>[2x]VTDLAGTTRLLRAQGVTAPAGFRAAGVAAGIKASGALDLALVFNEGPDYAAAGVFTRNQVKAAPVLWTQQVLTTGRLRAVILNSGGANACTGPAGFADTHATAEAVAAALSDWGTETGAIEVAVCSTGLIGDRLPMDKLLAGVAHVVH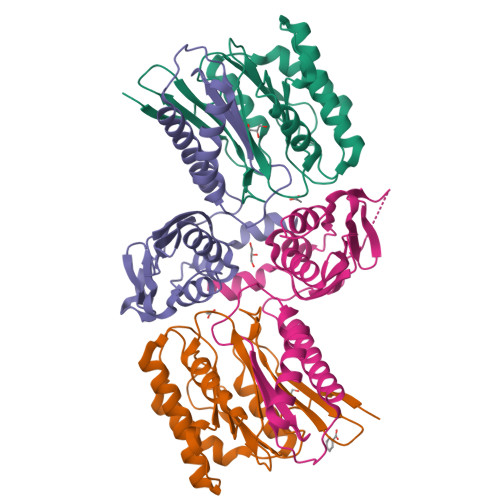EMHGGLVGGDEAAHAIMTTDNVPKQVALHHHDNWTVGGMAKGAGMLAPSLA;>TMLCVLTTDAAAEPAALERALRRAAAATFDRLDIDGSCSTNDTVLLLSSGASEIPPAQADLDEAVLRVCDDLCAQLQADAEGVTKRVTVTVTGAATEDDALVAARQIARDSLVKTALFGSDPNWGRVLAAVGMAPITLDPDRISVSFNGAAVCVHGVGAPGAREVDLSDADIDITVDLGVGDGQARIRTTDLSHAYVEENSAYSS[2x]(~{E})-6-[2-[3-[[(2~{R})-4-[[[(2~{R},3~{S},4~{R},5~{R})-5-(6-aminopurin-9-yl)-4-oxidanyl-3-phosphonooxy-oxolan-2-yl]methoxy-oxidanyl-phosphoryl]oxy-oxidanyl-phosphoryl]oxy-3,3-dimethyl-2-oxidanyl-butanoyl]amino]propanoylamino]ethylsulfanyl]-6-oxidanylidene-hex-3-enoic 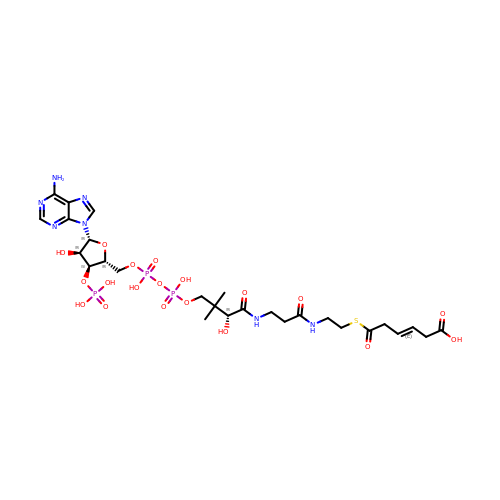acid | C27 H42 N7 O19 P3 S | VYSXESTVCZRDBA-ZPJAMBCCSA-N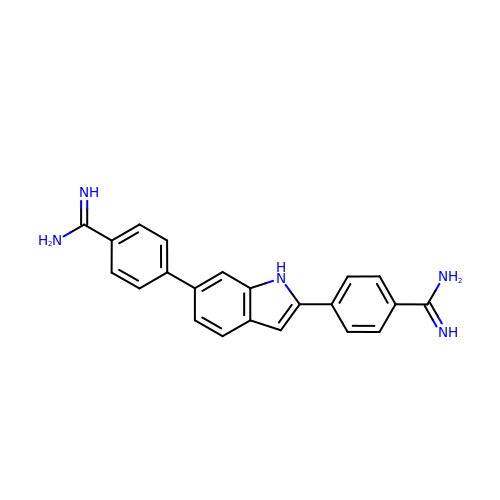4,4'-(1H-indole-2,6-diyl)dibenzenecarboximidamide | C22 H19 N5 | AXMNWOOVENPWID-UHFFFAOYSA-N> AIHEIKQNGNRYKIEKVTDSSLKQALASLRQSAWNVKELDLSGNPLSQISAADLAPFTKLELLNLSSNVLYETLDLESLSTLRTLDLNNNYVQELLVGPSIETLHAANNNISRVSCSRGQGKKNIYLANNKITMLRDLDEGCRSRVQYLDLKLNEIDTVNFAELAASSDTLEHLNLQYNFIYDVKGQVVFAKLKTLDLSSNKLAFMGPEFQSAAGVTWISLRNNKLVLIEKALRFSQNLEHFDLRGNGFHCGTLRDFFSKNQRVQTVAKQTVKKLTGQNEEECTVPTLGHYGAYCCEDLPAPFADRLIALKRKEHALLSGQGSETERLECERENQARQREIDALKEQYRTVIDQVTLRKQAKITLEQKKKALDEQVSNGRRAHAELDGTLQQAVGQIELQHATEEQSPLQLLRAIVKRYEEMYVEQQSVQNNAIRDWDMYQHKETQLAEENARLKKLNGEADLALASANATLQELVVREQNLASQLG;> VGGQQRYNVKPRQPEYKCIDSNLQYDCVFYDVHIDMQTQDVYFGFEDITLNNQKIVTFKNSTMRKLPAALLDSFRQ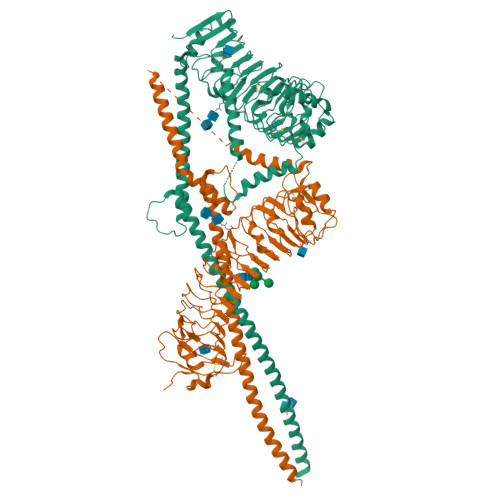VELLNLNDLQIEEIDTYAFAYAHTIQKLYMGFNAIRYLPPHVFQNVPLLTVLVLERNDLSSLPRGIFHNTPKLTTLSMSNNNLERIEDDTFQATTSLQNLQLSSNRLTHVDLSLIPSLFHANVSYNLLSTLAIPIAVEELDASHNSINVVRGPVNVELTILKLQHNNLTDTAWLLNYPGLVEVDLSYNELEKIMYHPFVKMQRLERLYISNNRLVALNLYGQPIPTLKVLDLSHNHLLHVERNQPQFDRLENLYLDHNSIVTLKLSTHHTLKNLTLSHNDWDCNSLRALFRNVARPAVDDADQHCKIDYQLEHGLCCKESDKPYLDRLLQYIALTSVVEKVQRAQGRCSATDTINSVQSLSHYITQQGGVPLQGNEQLEAEVNELRAEVQQLTNEQIQQEQLLQGLHAEIDTNLRRYRLPKDGLARSSDNLNKVFTHLKERQAFKLRETQARRTEADAKQKETEDLEQENIALEKQLDNKRAKQAELRQETSLKRQKVKQLEAKKNRNPDTRRVSHHHHHH E-AMINO BIOTINYL CAPROIC ACID | C16 H27 N3 O4 S 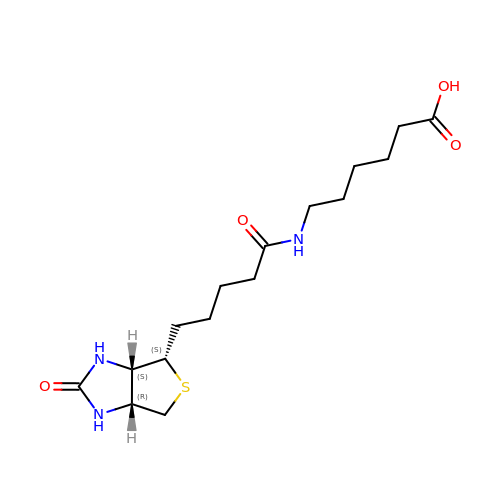| CMUGHZFPFWNUQT-HUBLWGQQSA-N>LDATPLSSPRHVRIKNWGSGMTFQDTLHHKAKGILTCRSKSCLGSIMTPKSLTRGPRDKPTPPDELLPQAIEFVNQYYGSFKEAKIEEHLARVEAVTKEIETTGTYQLTGDELIFATKQAWRNAPRCIGRIQWSNLQVFDARSCSTAREMFEHICRHVRYSTNNGNIRSAITVFPQRSDGKHDFRVWNAQLIRYAGYQMPDGSIRGDPANVEFTQLCIDLGWKPKYGRFDVVPLVLQANGRDPELFEIPPDLVLEVAMEHPKYEWFRELELKWYALPAVANMLLEVGGLEFPGCPFNGWYMGTEIGVRDFCDVQRYNILEEVGRRMGLETHKLASLWKDQAVVEINIAVLHSFQKQNVTIMDHHSAAESFMKYMQNEYRSRGGCPADWIWLVPPMSGSIT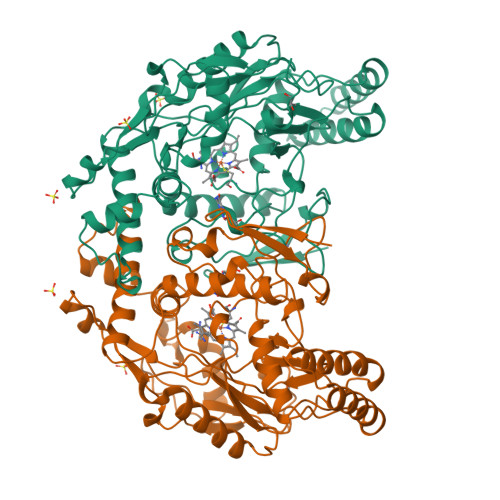PVFHQEMLNYVLSPFYYYQVEAWKTHVWQDE[4x]>[6x]MLEAQVQFASLWKRLVECINGLVNEANFDCNPGGLSVQAMDSSHVALVHMLLRDDCFVKYQCGRNSILGLNLASLSKVLKIVDSNDSLSLRHDDDSDVVTLTSENPEKTRKCEYQLKLLEIEAESMGIPEMDYRSTVTLNSAEFAK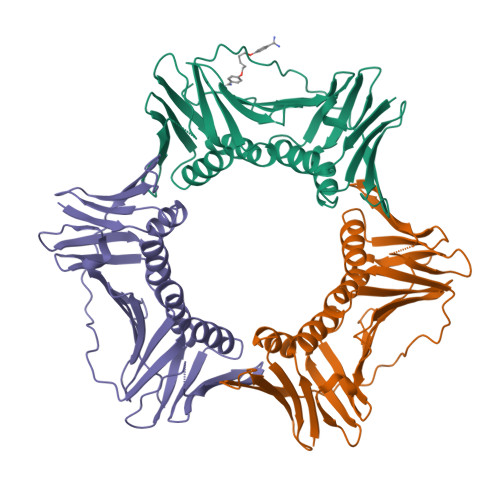IVRDMQVFGDTVTIAISKEGVKFSSSGDVGQGYTFLQAAGVSDRSTKSEVKAEVKAEARDDDEEPLSRKYGKADSSANAIGVEVTMEEPITLSFALRFMGIFAKGSTLSERVTLKFAKDSPCMVEYGIDNVGYLRYYLAPKVD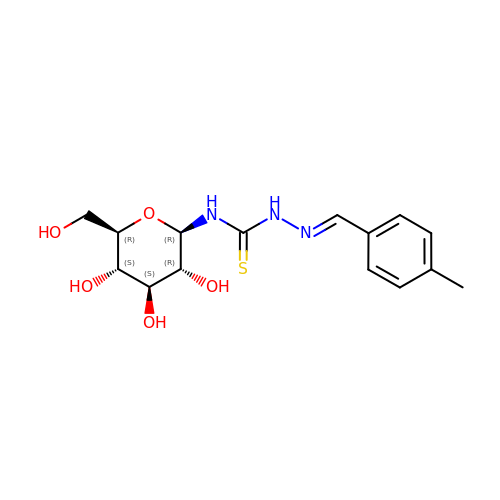N-({(2E)-2-[(4-methylphenyl)methylidene]hydrazino}carbonothioyl)-beta-D-glucopyranosylamine | C15 H21 N3 O5 S | DVGNOMWZPXETCK-VSZQLFBDSA-N PHOSPHONOACETIC ACID | C2 H5 O5 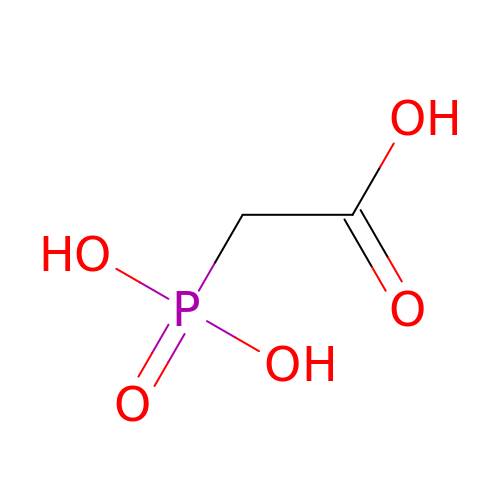P | XUYJLQHKOGNDPB-UHFFFAOYSA-N> NDQLVELAKDPANWVMTGRDYNAQNYSEMTDINKENVKQLRPAWSFSTGVLHGHEGTPLVVGDRMFIHTPFPNTTFALDLNEPGKILWQNKPKQNPTARTVACCDVVNRGLAYWPGDDQVKPLIFRTQLDGHIVAMDAETGETRWIMENSDIKVGSTL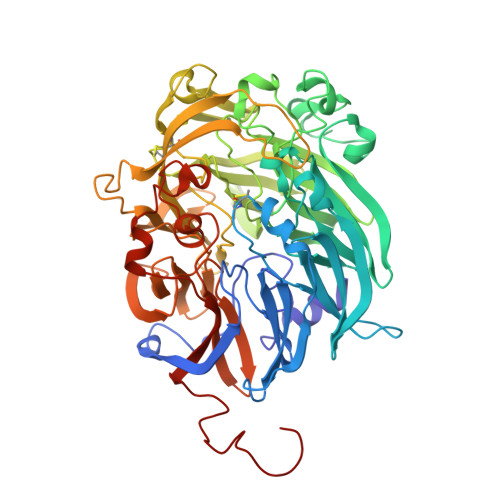TIAPYVIKDLVLVGSSGAELGVRGYVTAYDVKSGEMRWRAFATGPDEELLLAEDFNAPNPHYGQKNLGLETWEGDAWKIGGGTNWGWYAYDPEVDLFYYGSGNPAPWNETMRPGDNKWTMAIWGREATTGEAKFAYQKTPHDEWDYAGVNVMMLSEQEDKQGQMRKLLTHPDRNGIVYTLDRTNGDLISADKMDDTVNWVKEVQLDTGLPVRDPEFGTRMDHKARDICPSAMGYHNQGHDSYDPERKVFMLGINHICMDWEPFMLPYRAGQFFVGATLTMYPGPKGDRGNASGLGQIKAYDAISGEMKWEKMERFSVWGGTMATAGGLTFYATLDGFIKARDSDTGDLLWKFKLPSGVIGHPMTYKHDGRQYVAIMYGVGGWPGVGLVFDLADPTAGLGSVGAFKRLQEFTQMGGGVMVFSLDGESPYSDPNVGEYAPGEPT> AARKSAP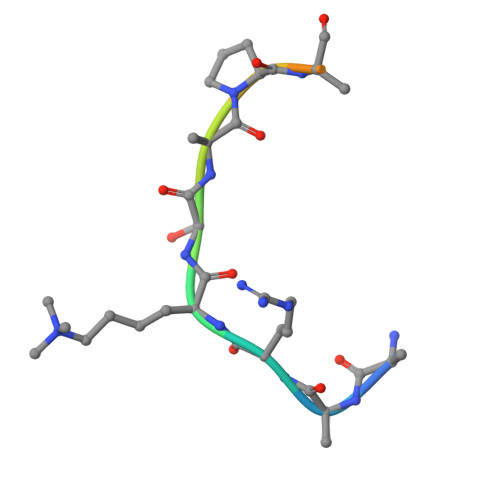ATGGV>MNKDQSKIPQATAKRLPLYYRFLKNLHASGKQRVSSAELSDAVKVDSATIRRDFSYFGALGKKGYGYNVDYLLSFFRKTLDQDEMTDVILIGVGNLGTAFLHYNFTKNNNTKISMAFDINESKIGTEVGGVPVYNLDDLEQHVK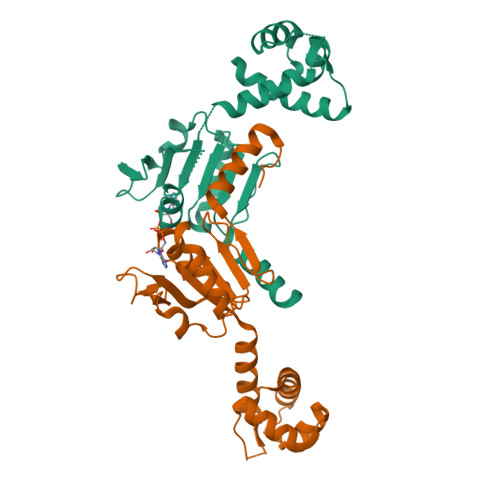DESVAILTVPAVAAQSITDRLVALGIKGILNFTPARLNVPEHIRIHHIDLAVELQSLVYFLKHYSVLEEIE[2x]> MVSDIVLEVQSLHVYYGAIHAIKGIDLKVPRGQIVTLIGANGAGKTTTLSAIAGLVRAQKG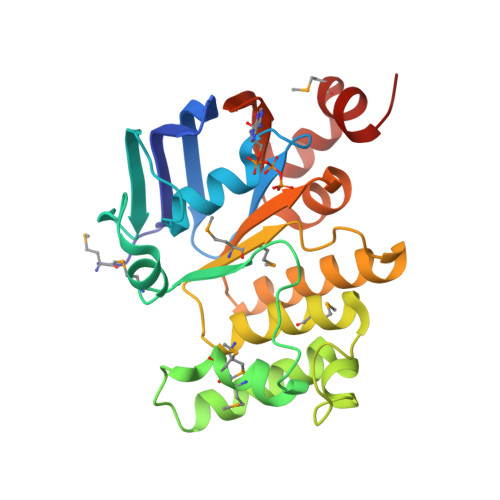KIIFNGQDITNKPAHVINRMGIALVPEGRRIFPELTVYENLMMGAYNRKDKEGIKRDLEWIFSLFPRLKERLKQLGGTLSGGEQQMLAIGRALMSRPKLLMMDEPSLGLAPILVSEVFEVIQKINQEGTTILLVEQNALGALKVAHYGYVLETGQIVLEGKASELLDNEMVRKAYLGVA> GSTLEDLFG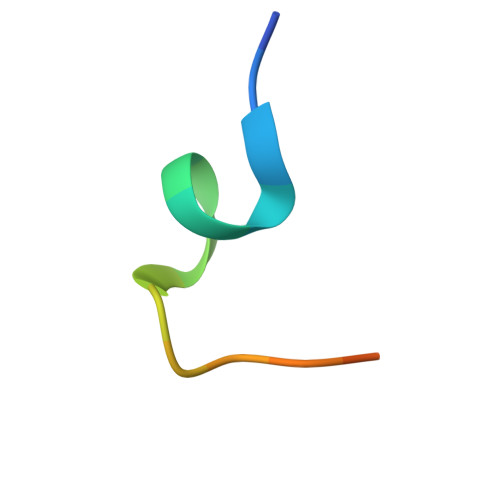PLFYVDKSL>MTLHKERRIGRLSVLLLLNEAEESTQVEELERDGWKVCLGKVGSMDAHKVIAAIETASKKSGVIQSEGYRESHALYHATMEALHGVTRGEMLLGSLLRTVGLRFAVLRGNPYESEAEGDWIAVSLYGTIGAPIKGLEHETFG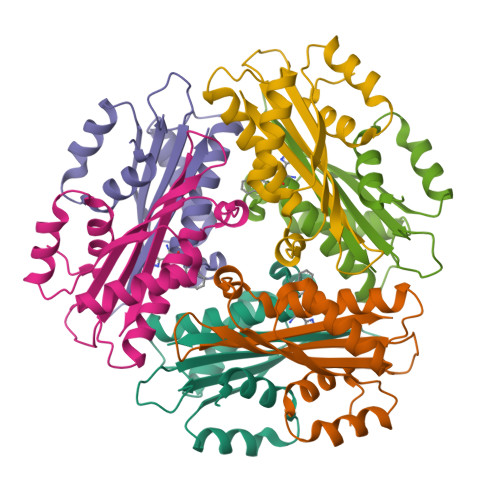VGINHI[2x]> XFAAAAG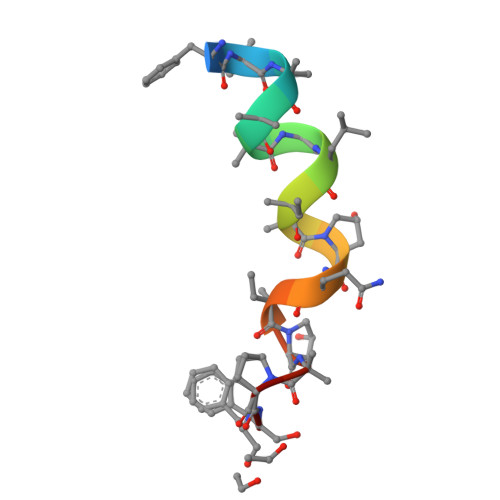LVAPQVPAPF>[2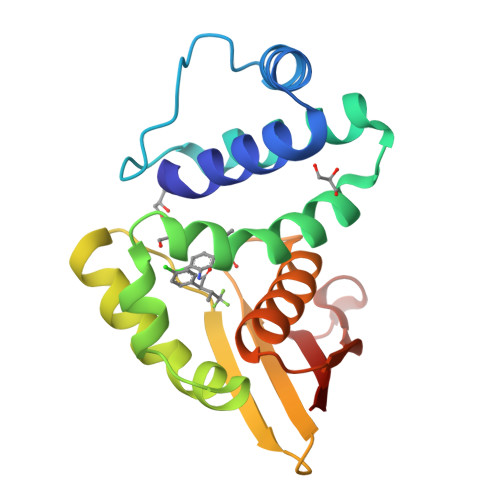x]MYGLVNKAIQDMISKHHGEDTWEAIKQKAGLEDIDFFVGMEAYSDDVTYHLVGAASEVLGKPAEELLIAFGEYWVTYTSEEGYGELLASAGDSLPEFMENLDNLHARVGLSFPQLRPPAFECQHTSSKSMELHYQSTRAGLAPMVLGLLHGLGKRFQTKVEVTQTAFRETGEDHDIFSIKYE>PSVYDAAAQLTADVKKDLRDSWKVIGSDKKGNGVALMT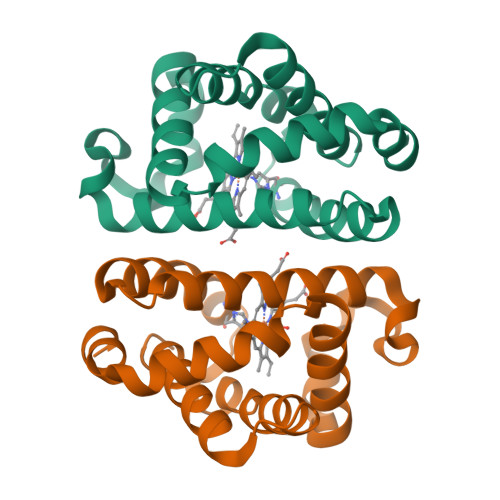TLFADNQETIGYFKRLGDVSQGMANDKLRGHSITLMYALQNFIDQLDNPDDLVCVVERFAVNHITRKISAAEFGKINGPIKKVLASKNFGDKYANAWAKLVAVVQAAL[4x]N-(phenylcarbonyl)-beta-D-glucopyranosylamine 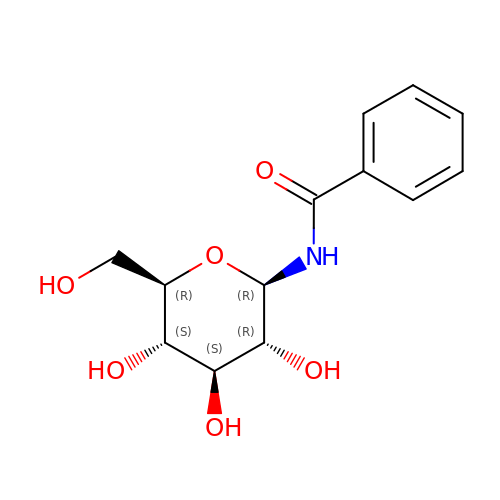| C13 H17 N O6 | SPYSOSUFGSNSMY-BZNQNGANSA-N(4~{R})-4-pyridin-3-yl-4,5-dihydropyrrolo[1,2-a]quinoxaline 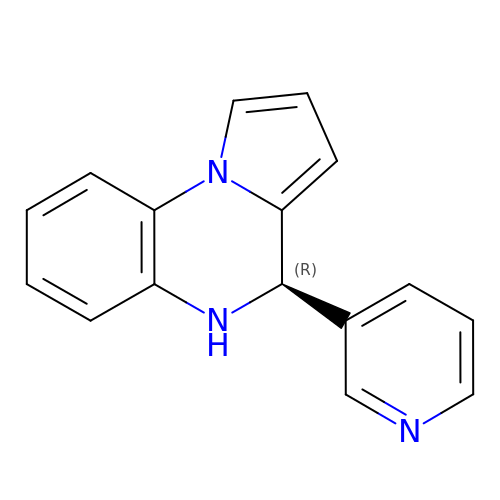| C16 H13 N3 | BSOBGTYXYGHUTD-MRXNPFEDSA-N>MAEIPKEMLRAQTNXILLNVLKQGDNYVYGIIKQVKEASNGEMELNEATLYTIFKRLEKD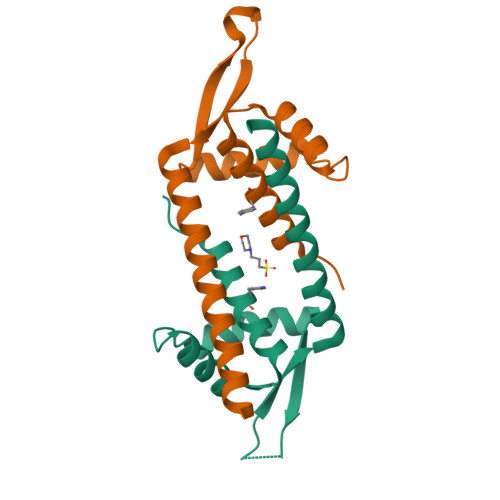GIISSYWGDESQGGRRKYYRLTEIGHENMRLAFESWSRVDKIIENLEANKKSEAIKSRWSHPQFEK[2x]>[2x]MLNRVVLVGRLTKDPELRSTPNGVNVGTFTLAVNRTFTNAQGEREADFINVVVFKK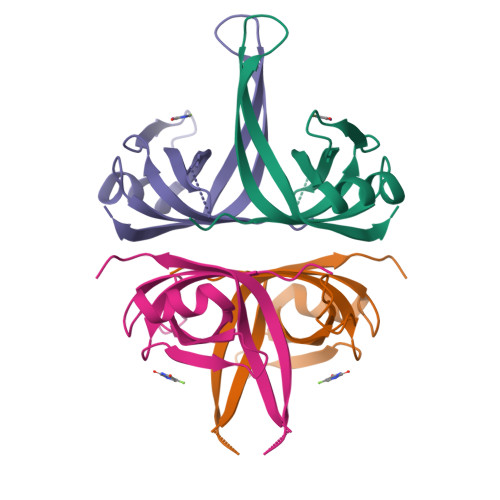QAENVKNYLSKGSLAGVDGRLQTRNYENKDGQRVFVTEVVADSVQFLEPKHHHHHH The t6A biosynthesis pathway consists of two steps: firstly, the YRDC enzyme (Sua5 in yeast) synthesizes an unstable threonylcarbamoyl-AMP intermediate (TC-AMP) and in a second step, the KEOPS protein complex transfers the TC-moiety from TC-AMP onto the tRNA substrate. The eukaryotic KEOPS complex contains five subunits GON7/LAGE3/OSGEP/TP53RK/TPRKB that are arranged linearly in that order. OSGEP is the catalytic subunit that carries out the TC-transfer reaction and its orthologs are present in virtually all sequenced genomes. The other subunits are essential for the t6A modification of tRNA, but their precise roles are as yet unknown, especially that of GON7, an intrinsically disordered protein (IDP), which was only recently identified in humans.

Furthermore, we determine the crystal structure of the GON7/LAGE3/OSGEP KEOPS subcomplex showing that GON7 becomes structured upon binding to LAGE3. We obtained 1.9 Å resolution diffraction data of the GON7/LAGE3/OSGEP complex. LAGE3 is at the center of the complex, binding on one side to OSGEP and on the other to GON7, which does not directly interact with OSGEP. The two helices of LAGE3 associate with the N-terminal helices of OSGEP into a helical bundle. Only 45% of the GON7 sequence adopts a well-defined structure upon binding to LAGE3, confirming our SAXS- and NMR-based conclusions. The N-terminal peptide of GON7 forms a β-hairpin between Met1 and Ser20 and the region between Gly25 and Pro50 forms a helix that lies parallel against the β-hairpin. The β-hairpin of GON7 aligns with the β-sheet of LAGE3 to form a continuous five stranded anti-parallel sheet. The helix of GON7 packs in an anti-parallel orientation against the C-terminal helix of LAGE3. The association mode between GON7 and LAGE3 is very similar to that of the yeast Pcc1/Gon7 complex, illustrated by their superposition (RMSD = 1.4 Å).

> MRDADADAGGGADGGDGRGGHSCRGGVDTAAAPAGGAPPAHAPGPGRDAASAARGSRMRPHIFTLSVPFPTPLEAEIAHGSLAPDAEPHQRVVGKDLTVSGRILVVRWKAEDCRLLRISVINFLDQLSLVVRTMQRFGPPVSR;> MELLGEYVGQEGKPQKLRVSCEAPGDGDPFQGLLSGVAQMKDMVTELFDPLVQGEVQHRVAAAPDEDLDGDDEDDAEDENNIDNRTNFDGPSAKRPKTPSHHHHHH;> MPAVLGFEGSANKIGVGVVRDGKVLANPRRTYVTPPGTGFLPGDTARHHRAVILDLLQEALTESGLTSQDIDCIAYTKGPGMGAPLVSVAVVARTVAQLWNKPLVGVNHCIGHIEMGRLITGATSPTVLYVSGGNTQVIAYSEHRYRIFGETIDIAVGNCLDRFARVLKISNDPSPGYNIEQMAKRGKKLVELPYTVKGMDVSFSGILSFIEDVAHRMLATGECTPEDLCFSLQETVFAMLVEITERAMAHCGSQEALIVGGVGCNVRLQEMMATMCQERGARLFATDERFCIDNGAMIAQAGWEMFRAGHRTPLSDSGVTQRYRTDEVEVTWRD> TLRDTIPDCALRSQTLESLDARYVS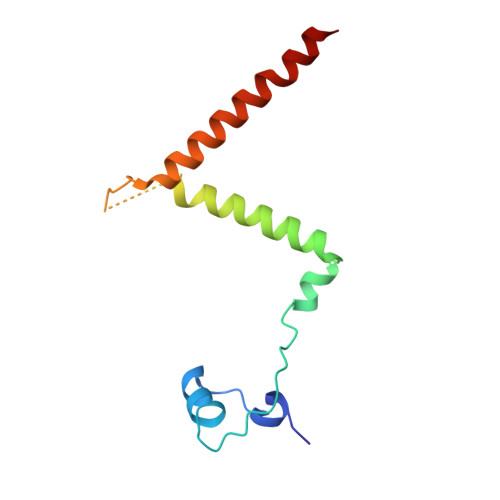RDGAHDAAVWFEDMTPAELEVVFPTTDAKLNYLSRTQRLASLLTYAGPIKAPDDAAAPQTPDTACVHGELLARKRERFAAVINRFLDLHQILR>[2x]MHSAANAKQQKHFVLVHGGCLGAWIWYKLKPLLESAGHKVTAVDLSAAGINPRRLDEIHTFRDYSEPLMEVMASIPPDEKVVLLGHSFGGMSLGLAMETYPEKISVAVFMSAMM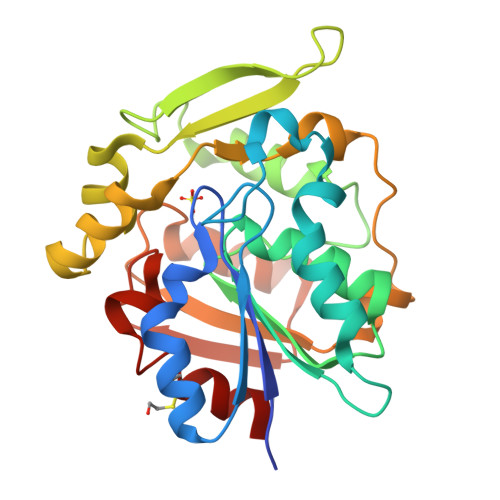PDPNHSLTYPFEKYNEKCPADMMLDSQFSTYGNPENPGMSMILGPQFMALKMFQNCSVEDLELAKMLTRPGSLFFQDLAKAKKFSTERYGSVKRAYIFCNEDKSFPVEFQKWFVESVGADKVKEIKEADHMGMLSQPREVCKCLLDISDS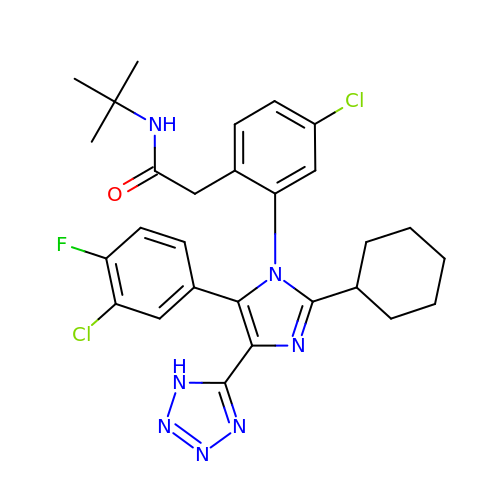~{N}-~{tert}-butyl-2-[4-chloranyl-2-[5-(3-chloranyl-4-fluoranyl-phenyl)-2-cyclohexyl-4-(1~{H}-1,2,3,4-tetrazol-5-yl)imidazol-1-yl]phenyl]ethanamide | C28 H30 Cl2 F N7 O | SFBXQXHCYMXGGU-UHFFFAOYSA-N> HKSIKEIEKEEIIKVLKEVNFNKKLASEILGIPLRTLYKR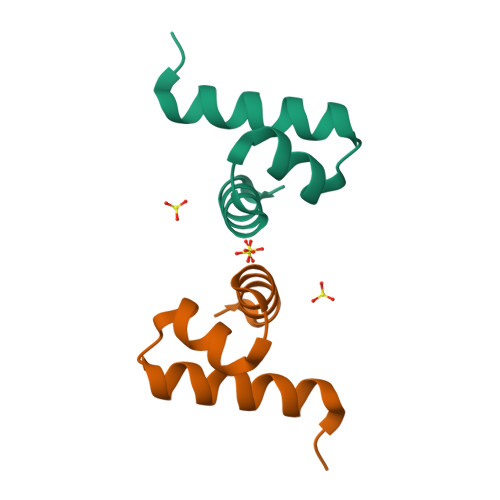LKEYGI>[2x]MTWLPLNPIPLKDRVSMIFLQYGQIDVIDGAFVLIDKTGIRTHIPVGSVACIMLEPGTRVSHAAVRLAAQVGTLLVWVGEAGVRVYASGQPGGARSDKLLYQAKLALDEDLRLKVVRKMFELRFGEPAPARRS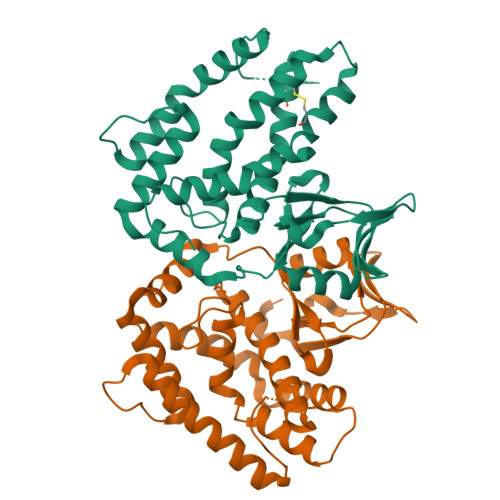VEQLRGIEGSRVRATYALLAKQYGVTWNGRRYDPKDWEKGDTINQCISAATSCLYGVTEAAILAAGYAPAIGFVHTGKPLSFVYDIADIIKFDTVVPKAFEIARRNPGEPDREVRLACRDIFRSSKTLAKLIPLIEDVLAAGEIQPPAPPEDAQPVAIPLPVSLGDAGHRSS> MVKLRDWQEKLKDKVIEGLRNNFLVALNAPTGSGKTLFSLLVSLEVKPKVLFVVRTHNEFYPIYRDLTKIREKRNITFSFLVGKPSSCLYAEKGAESEDIPCKYCELKGSIVEVKTDDSPLSLVKKLKKDGLQDKFCPYYSLLNSLYKADVIALTYPYFFIDRYREFIDIDLREYMIVIDEAHNLDKVNELEERSLSEITIQMAIKQSKSEESRRILSKLLNQLREVVLPDEKYIKVENVPKLSKEELEILADDYEDIRKDSLKQGKVNKIHIGSILRFFSLLSIGSFIPFSYSKRLVIKNPEISYYLNLLNDNELSIILMSGTLPPREYMEKVWGIKRNMLYLDVERE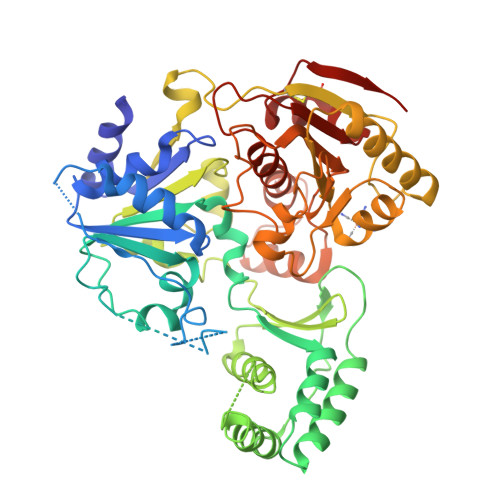IQKRVSGSYECYIGVDVTSKYDMRSDNMWKRYADYLLKIYFQAKANVLVVFPSYEIMDRVMSRISLPKYVESEDSSVEDLYSAISANNKVLIGSVGKGKLAEGIELRNNDRSLISDVVIVGIPYPPPDDYLKILAQRVSLKMNRENEEFLFKIPALVTIKQAIGRAIRDVNDKCNVWLLDKRFESLYWKKNLKCLNANKMKL> VDAGLDQIENREVLRPLLEALPERERTVLVLRFFDSMTQTQIAER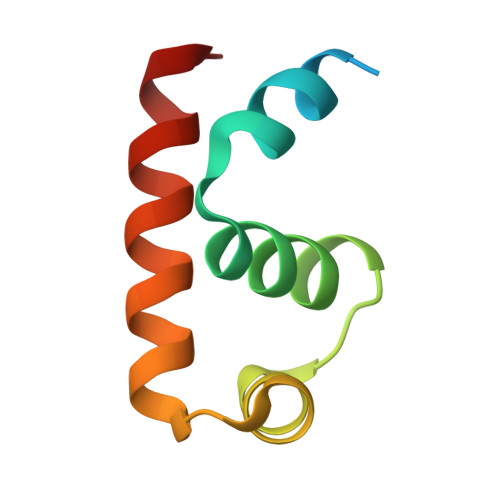VGISQMHVSRLLAKSLARLRDQLE>KVDPNKIYTIDEAAHLVKELATAKFDETVEVHAKLGIDPRRSDQNVRGTVSLPHGLGKQVRVLAIAKGEKIKEAEEAGADYVGGEEIIQKILDGWMDFDAVVATPDVMGAVGSKLGRILGPRGLLPNPKAGTVGFNIGEIIREIKAGRIEFRNDKTGAIHAPVGKASFPPEKLADNIRAFIRALEAHKPEGAKGTFLRS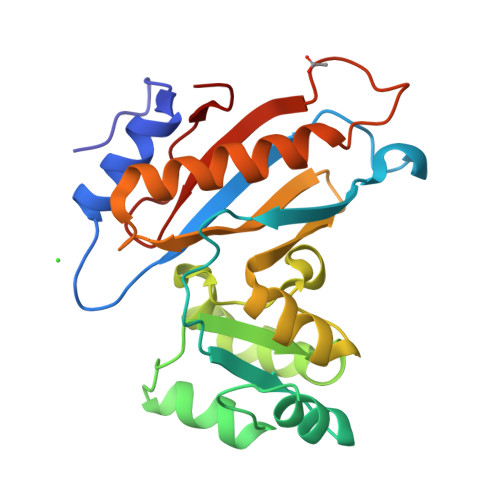VYVTTTMVPSVRINPHS[2x]>[2x]MPQLHYVPYDTPVEDVMRILKESGTLVIRNFLDQNTVQKVQDEVDDYVRNWNPGPKYNHDIKTVGSKTKQPSNLSLMSKTYRCEVLNHPWMHAICERMFGPTYGDYWFNGGSILHLEPGENTQPIHQDHVFYQISKWRRPTDPDLTINFTMALTEFTVENGGTRVCPGSHLWENGHASPAEEDMVPVLMQPGDALILP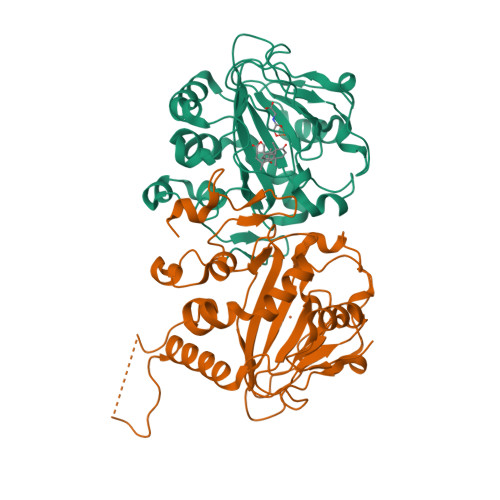GSMWHSAGANRTSEYRRGFATSFHPCHFTPIESHHHLPREMVEEMTPLVQKMLGFRTLNLHNNVKVWKAGEGNLEDATGLKSVAAKLAAALEHHHHHH> GTGGGCCGAC;> GTCGG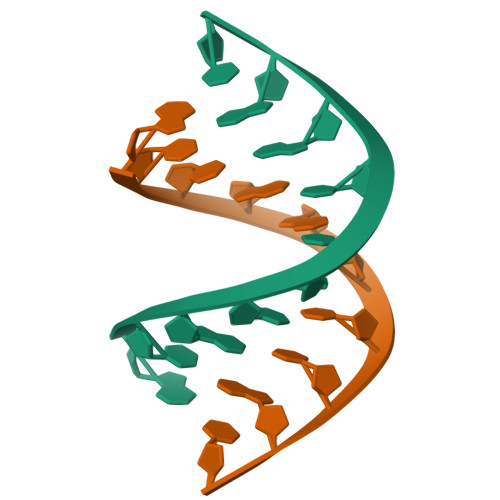CCCAC>[2x]QEPQPEQDPFELSGKWITSYIGSSDLEKIGENAPFQVFMRSIEFDDKESKVYLNFFSKENGICEEFSLIGTKQEGNTYDVNYAGNNKFVVSYASETALIISNINVDEEGDKT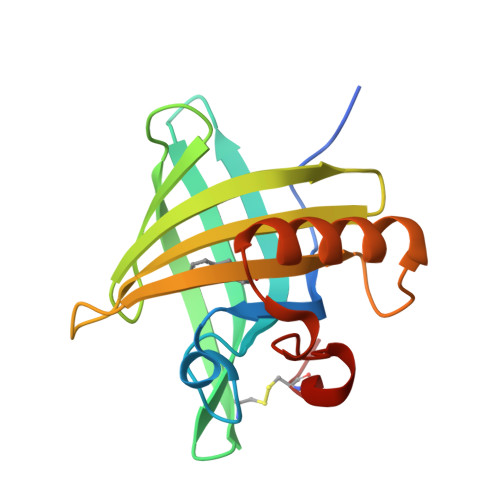IMTGLLGKGTDIEDQDLEKFKEVTRENGIPEENIVNIIERDDCPA> GSHMSNTQTVLPFTGLNTPSGVAVDSAGT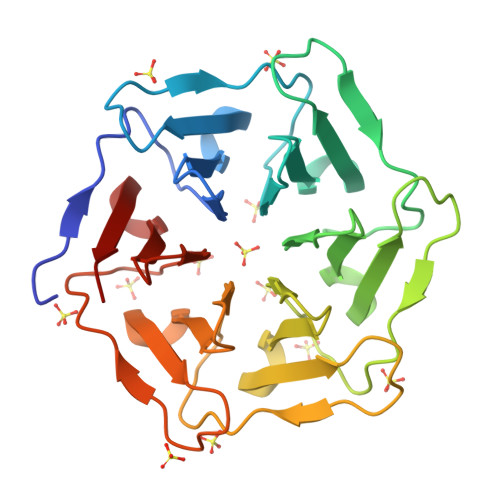VYVTDHGNNRVVKLAAGSTNQVTLPFTGLNTPHGVAVDSAGTVYVTDHGNNRVVKLAAGSNTQTVLPFTGLNTPSGVAVDSAGTVYVTDHGNNRVVKLAAGSTNQVTLPFTGLNTPHGVAVDSAGTVYVTDHGNNRVVKLAAGSNTQTVLPFTGLNTPSGVAVDSAGTVYVTDHGNNRVVKLAAGSTNQVTLPFTGLNTPHGVAVDSAGTVYVTDHGNNRVVKLAAG2-[4-[[4-[4-(4-ethanoyl-3-ethyl-5-methyl-1~{H}-pyrrol-2-yl)-1,3-thiazol-2-yl]piperazin-1-yl]methyl]-1,2,3-triazol-1-yl]ethanamide 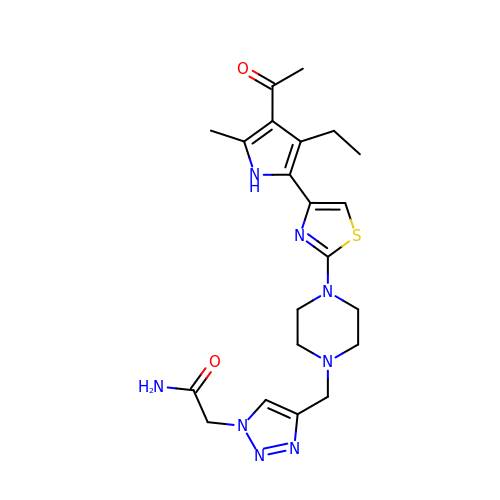| C21 H28 N8 O2 S | JHPCBFLUKPVPEM-UHFFFAOYSA-N V1 is a part of an ion pump V-ATPase, which transports cations across the membrane by ATP-hydrolysis-driven rotation. V1 comprises a rotor composed of the D and F subunits, and a stator, a hexameric ring, composed of three A subunits and three B subunits. However, the details of their sequences and structures are different, resulting in two different interfaces between the A and B subunits in the A3B3 hexameric ring: a catalytic interface, at which the A subunit has an ATP-hydrolysis catalytic site; and a non-catalytic interface, at which the B subunit has a pseudo-active site, which has evolutionally lost the ATP-hydrolysis or even binding ability. We used computational design to restore the lost ATP-binding ability of the pseudo-active site in the B subunit of a rotary molecular motor, V1-ATPase.

To provide a structure-based interpretation of the allosteric effect, two additional crystal structures were solved. The nucleotide-free crystals were incubated overnight by gradually increasing the ADP concentration to 5 mM, and two different structural states in an asymmetric unit were obtained from one dataset at 4.2 Å resolution. Comparison of the two structures indicates that a nucleotide binding to the designed site induces the movement of the C-terminal α-helical domains of the designed B subunit and neighbour A subunit, which changes the conformation of the neighbouring catalytic interface from closed to open-like. The conformational change expands the space around the catalytic site formed between the α/β domains of the designed B subunit and neighbour A subunit. This probably weakens the interactions of the catalytic site with ADP. The conformational change suggests a structural mechanism for the facilitation of ADP release at the catalytic sites upon the ATP binding to the designed sites, although the structures are bound with ADP not ATP and do not contain the rotor subunits. The solved crystal structures suggest that the allosteric effect occurs upon the transition of the nucleotide occupation number for the designed sites from one to two. It should be noted, in particular, that the three designed nucleotide-binding sites have different binding affinities because not all of them were occupied by nucleotide in the solved crystal structures.

>[6x]SSGMQIGKIIKVSGPLVMAENMSEASIQDMCLVGDLGVIGEIIEMRQDVASIQVYEETSGIGPGEPVRSTGEALSVELGPGIISQMFDGIQRPLDTFMEVTQSNFLGRGVQLPALDHEKQWWFEATIEEGTEVSAGDIIGYVDETKIIQHKIMVPNGIKGTVQKIESGSFTIDDPICVIETEQGLKELTMMQKWPVRRGRPIKQKLNPDVPMITGQRVIDTFFPVTKGGAAAVPGPFGAGKTVVQHQIAKWSDVDLVVYVGCGERGNEMTDVVNEFPELIDPNTGESLMERTVLIANTSNMPVAAREASIYTGITIAEYFRDMGYDVAIMADSTSRWAEALREMSGRLEEMPGDEGYPAYLGSRLAEYYERSGRVIALGSDQREGSITAISAVSPSGGDISEPVTQNTLRVVKVFWGLDSSLAQKRHFPSINWIQSYSLYSTEVGRYMDQILQQDWSDMVTEGMRILQEEEQLNEIVRLVGIDSLSDNDRLTLEVAKSIREDYLQQNAFDDVDTFTSREKQFNMLKVILTFGKEARKALSLGAYFNEIMEGTVAVRERISRSKYIPEEELAKISSINEEIKETIQLIVSEGGMTDD;>MIKEYRTIKEVVGPLMAVEKVSGVKYEELIEVRMQNGEIRRGQVLEVQEDKAMVQIFEGTSGINLKNSSVRFLGHPLQLGVSEDMIGRVFDGLGRPKDNGPEILPEKYLDINGEVINPIARDYPDEFIQTGISAIDHLNTLVRGQKLPVFGPPGAGKSALAAQIARQATVLDSSDDFAVVFAAIGITFEEAEFFMEDFRQTGAIDRSVMFMNLANDPAIERIATPRMALTAAEYLAYEKGMHVLVIMEDMTNYAEALREISAARREVPGRRGYPGYLYTNLATLFERAGRIRGLKGSVTQIPILTMPEDDKTHPIPDLTGYITEGQIILTRELYKSGISPPIDVLPSLSRLKDKGTGAGKTREDHAATMNQLFAAYAQGKQAKELAVVLGESALSDIDKIYAKFAERFENEYVNQGFYTNRTITETLDLGWELLAMLPRTELKRIKDDLLDKYLPEGK[6x]>MSLAHTAAEYMLS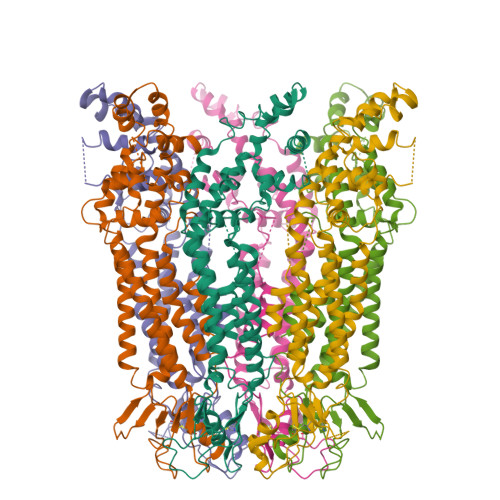DALLPDRRGPRLKGLRLELPLDRIVKFVAVGSPLLLMSLAFAQEFSSGSPISCFSPSNFSIRQAAYVDSSCWDSLLHHKQDGPGQDKMKSLWPHKALPYSLLALALLMYLPVLLWQYAAVPALSSDLLFIISELDKSYNRSIRLVQHMLKIRQKSSDPYVFWNELEKARKERYFEFPLLERYLACKQRSHSLVATYLLRNSLLLIFTSATYLYLGHFHLDVFFQEEFSCSIKTGLLSDETHVPNLITCRLTSLSIFQIVSLSSVAIYTILVPVIIYNLTRLCRWDKRLLSVYEMLPAFDLLSRKMLGCPINDLNVILLFLRANISELISFSWLSVLCVLKDTTTQKHNIDTVVDFMTLLAGLEPSKPKHLTNSACDEHP[6x]>MHHHHHHGSGSGSSVLQVLTFPDDRLRTVAKPVEQVTPEIQQIVDDMLETMYAEEGIGLAATQVDIHQRIVVIDISETRDQPMVLINPEIIEKRGEDGIEEGCLSVPGARALVPRAAEVTVKALDRNGQEYQFDADDLLAICVQHELDHLAGKLFVDYLSPLKRNRIKEKLEKIKRFNEKK[2x]

Peptide deformylases (PDFs) are metalloproteases that catalyze the removal of the formyl group from the initiator methionine, a critical step in the N-terminal methionine excision (NME) process. Most PDFs share a common catalytic core defined by three conserved sequence motifs (I, II, and III), which coordinate a metal ion and position key residues for substrate processing. All peptide-based PDF inhibitors share a common mechanism of action: they bind to the catalytic pocket of the enzyme, thereby preventing substrate access and inhibiting its deformylase activity. Furthermore, our investigation of V. cholerae, which encodes two type 1b PDFs with 50% sequence homology (Def1VCH and Def2VCH), demonstrated that both PDFs are catalytically active.

The canonical PDF, Def1VCH, is located on chromosome 1 within an operon that includes fmt, rsmB, trkA (as in E. coli), trkH, and a gene of unknown function with a conserved DUF3157 domain (VC0041). In Def1VCH, all amino acids crucial for ribosome binding are identical to E. coli PDF, while in Def2VCH, R153 is substituted by a methionine and R163 by a lysine. To explore this possibility at the molecular level, we determined high-resolution crystal structures of both proteins in complex with ACT. In both structures, ACT binds in the same location within the catalytic pocket and adopts a nearly identical orientation and conformation, blocking access to the active site located at the bottom of a deep cavity in the protein core. In Def1VCH, all previously identified amino acids involved in ACT binding in E. coli PDF were also identified interacting with ACT. Additionally, in the hydrophobic pocket containing the ACT P1' aliphatic chain, isoleucine at position 86 and leucine at position 125 in Def1VCH are substituted by glycine and phenylalanine, respectively, in Def2VCH. Substitution of arginine 97 with tyrosine in Def1VCH resulted in a significant increase in the MIC to ACT, reaching levels comparable to those conferred by Def2VCH. Substitutions of glutamate 87 to glutamine (E87Q) and leucine 125 to phenylalanine (L125F) in Def1VCH had either no or intermediate effects, in the same direction as the R97Y substitution, and their effects appeared to be cumulative. Deletion of the canonical PDF def1VCH did not impact the sensitivity to ACT, but the deletion of the accessory PDF def2VCH led to a 20-fold decrease in the MIC of ACT.> MLYRGLRMAARAAPKFAVLNTHAALRQLPLQFQHVRTYADKIIKVPQMAESITEGTLKQWNKAVGDYVEADEEIATIETDKIDVAVNAPEAGVIKEFFVNEEDTVLVGQDLVRLEVGGEKPAEAAKEQPKAAAPEPKVEEKKVPEAPAPEPSKTAAPAPAPPKQEAPASPKPASKPAETPAVTLGNREERRVKMNRMRLRIAERLKQSQNTAASLTTFNEVDMSALIEFRNKYKDEVLKKTGVKLGFMSAFSRAVVLAIRDLPVVNASIEGPNGGDTIVYRDYVDISVAVATEKGLVTPVVRNAETMDLITIEKTIAELGKKARDGKLTIEDMAGGTFTISNGGVFGSLMGTPIINLPQSAVLGLHAIKERPVAVNGKVEIRPMMYLALTYDHRLLDGREAVQFLVKVKEYIEDPRKMLL

The oxoglutarate dehydrogenase complex (OGDHc) participates in the tricarboxylic acid cycle and, in a multi-step reaction, decarboxylates α-ketoglutarate, transfers succinyl to CoA, and reduces NAD+. At the molecular level, OGDHc is a megadalton-size assembly of multiple copies of three enzymes, namely E1o (oxoglutarate dehydrogenase, EC 1.2.4.2), E2o (dihydrolipoyl succinyltransferase, EC 2.3.1.61) and E3 (dihydrolipoyl dehydrogenase, EC 1.8.1.4). E2o forms the core of the complex with a stable stoichiometry of 24 copies in a cubic assembly, whereas the E1o and E3 proteins assemble on its periphery to carry out the complete reaction in a yet stoichiometrically and structurally unknown high-order metabolon. In addition, the lipoyl domain (LD) that transfers lipoyl intermediates from one active site to the next (E1o → E2o → E3) is part of a highly flexible E2o arm, representing a particular challenge for its study by traditional structural methods.

We further report the high-resolution cryo-EM structure of the OGDHc core (E2o), which displays various structural adaptations. The EM map displays higher-order structural features, e.g., inter-, and intra- trimeric interfaces, captures secondary structure elements and accurately places amino-acid side chains. We were able to identify the E2o’s catalytic active site and fully model side-chain conformations of the amino-acids participating in CoA binding which are conserved across oxo-acid dehydrogenases. F247 has an outward-facing orientation to accommodate the CoA, interacting and stabilizing the CoA 3’,5’-adenosine diphosphate group via π-stacking. The limited presence of electron density for the CoA pantoic acid, β-alanine, and cysteamine components underlies the inherent flexibility of endogenously bound coenzyme A with implications for function. A major difference lies in the fact that, compared to bacterial PDHc, which could be trapped in a proposed resting state with all LDs bound to the E2 active sites, the present eukaryotic OGDHc highlights an alternative resting state where LDs are sub-stoichiometrically and transiently interacting with the E2 core. By contrast, in C. thermophilum this element obtains a β-strand (E188-M194) conformation which, along with a β-hairpin motif of residues N266 - D282 creates an extended β-sheet. This adaptation contributes to the stabilization of the core via extensive hydrogen bonding and affects subunit inter-communication in the higher-order state of the 24-meric cubic E2o core. In line with this notion, C. thermophilum intra- and inter-subunit interfaces are 1.7 and 1.5 times larger than the corresponding interfaces of the human E2o core and include extensive charge-charge interactions.>MLIKKALTAVALLASLLGASAAFAHAHLKSATPAADSTVAAPADLRLTFSEGVEATFTKVSLSKDGTEVAIKGLETPDADKKTLVVTPAAPLA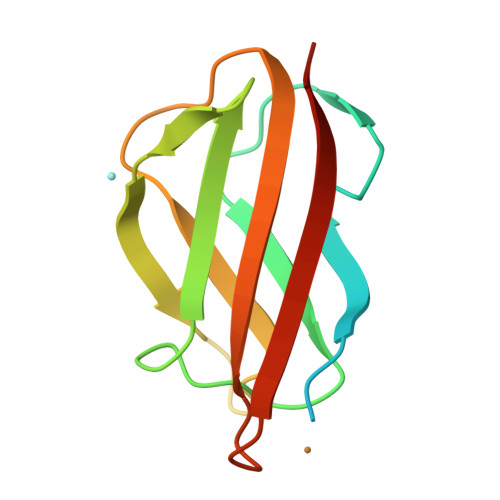AGNYKVVWNAVSVDTHKSNGEYSFKVKKK[3x]> AATTVNGGTVHFKGEVVNAACAVDAGSVDQTVQLGQVRTASLAQEGATSSAVGFNIQLNDCDTNVASKAAVAFLGTAIDAGHTNVLALQSSAAGSATNVGVQILDRTGAALTLDGATFSSETTLNNGTNTIPFQARYFATGAATPGAANADATFKVQYQ

The FimA subunits of the pilus rod are single domain proteins of 16 kDa with an incomplete, immunoglobulin (IG)2-like fold that lacks the C-terminal β-strand (G-strand). In the structure of the pilus rod, the FimA subunits interact via inter-molecular donor strand complementation, in which the N-terminal extension of each subunit, termed the donor strand, inserts as a β-strand into the preceding subunit and completes its IG-like fold. In 2010, Sukumaran et al. discovered that the FimA proteins from the enteroinvasive pathogens E. coli, Shigella flexneri, and Salmonella enterica have a second function besides formation of homopolymeric pilus rods; soluble forms of FimA, independent of FimC, act as inhibitors of host cell apoptosis after pathogen internalization by stabilizing the interaction between hexokinase and the voltage-dependent anion channel (VDAC) on the surface of mitochondria. We showed that all three FimA orthologues investigated (FimAECO, FimASHI, and FimASAL) were capable of folding to an alternative, self-complemented, monomeric form of only marginal thermodynamic stability that likely represents the FimA species that acts as an inhibitor of host cell apoptosis after internalization of the respective pathogen.

FimAECO, FimASHI, and FimASAL were produced as reduced, insoluble proteins in the E. coli cytoplasm without their N-terminal signal sequences. All proteins were refolded in the absence of the chaperone FimC under oxidizing conditions to allow the formation of the single, invariant structural disulfide bond. The purified proteins were crystallized, and their X-ray structures were determined at 1.5, 0.89, and 1.69 Å resolution, respectively. All FimA orthologues crystallized as self-complemented monomers, and all structures strongly resembled the previously reported NMR structure of the FimAECO monomer. The Cα RMSD between the most representative model of the self-complemented FimAECO NMR structure (2M5G, model 10, calculated with OLDERADO server) and FimAECO X-ray structure was 0.84 Å. In contrast to the intermolecular donor strand complementation (antiparallel to the FimA F-strand) observed for the assembled E. coli pilus rod, where the FimA side chains of Gly8, Val10, Phe12, Gly14, and Val16 from the donor strand occupy the binding pockets P1–P5 of the FimA-fold, the reversed (parallel) donor strand orientation in X-ray structure of self-complemented FimAECO showed the side chain occupancies P1/Gly14, P2/Phe12, P3/Val10, and P4/Gly8 (amino acid numbering according to E. coli FimA). Due to a lack of electron density, the occupancy of P5 with Val16, previously identified in the NMR structure of FimAECO, could not be confirmed in the X-ray structure, but the two structures otherwise proved to be essentially identical.>[2x]GPGVCKSYKSVALVVGVTGIVGSSLAEVLKLPDTPGGPWKVYGVARRPCPVWLAKKPVEYIQCDVSNNQETISKLSPLKDITHIFYVSWIGSEDCQTNATMFKNILNSVIPNASNLQHVCLQTGIKHYFAIFEEGSKVVPHDSP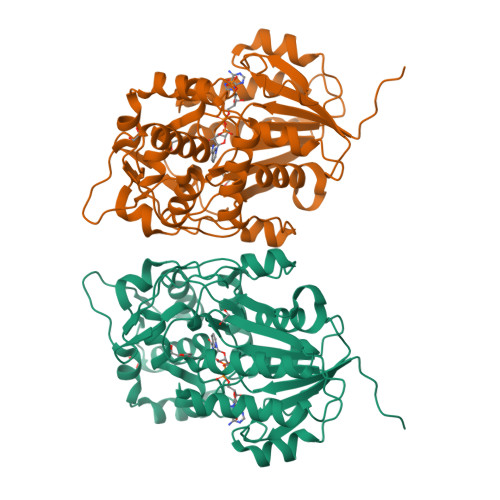FTEDLPRLNVPNFYHDLEDILYEETGKNNLTWSVHRPALVFGFSPCSMMNIVSTLCVYATICKHENKALVYPGSKNSWNCYADAVDADLVAEHEIWAAVDPKAKNQVLNCNNGDVFKWKHIWKKLAEEFGIEMVGYVEGKEQVSLAELMKDKDQVWDEIVKKNNLVPTKLKEIAAFWFADIAFCSENLISSMNKSKELGFLGFRNSMKSFVSCIDKMRDYRFIP> MKITNKSVDKQHIEKLDELRKNVSCTVIGFAEQTAELQQEISELFIAEFGVNGPIDMNSLSKLARITSYYASSEYFQGLAKYQRTACKMFITWQTLRKEAMECRSKDREIFASIPAKLCFFYFYNGELCRAVVCLLDYIDLSDDTLAKEAALRWLMFLGETELIEKKLKTWKMDKSSKDMFSATEFAMNYLKKSEYRVEMLEKLMKLRDKVKSDPTRSFSRYELASYVSWLCSTLSNVPVGSALRECEFPDRVSHIQEAALKSDSLVRNRIPGLASSQFDNSVNASIWPFLDGHQEDSNYYVHIGSTIAWHFEMRRECALVNVTTAQTRDSMSAMILNLRVALKSASFFRVLQTTNTLAYYSSIIEEAGSEK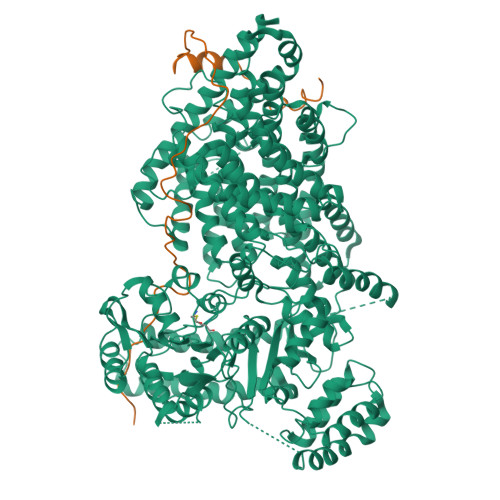NAKLMRVSCVNLLSSNPIIVRCSTPKETGATSRAHTPMAGSSVSEKQNTMRPDLADLLGDLELLDEQSFHPITRSCVCNVCTIYPLHSSFAAEYMMSYAIHSDFSQLSIKHFNDEFARIRERGMSSQVLMHRDSSVRPRPNIIQNEIFGMCVIRWLTKKLDSKESADEDTMEIFNNALKIVRYLQQRTTDMILAVTQLGRQLEFPMECNYSWMRPTIRKPRVKATIDCAVDILRAVSPFGRRPKVEKLEKNLQPFDKERFEKVRLAMRNEMNHYGHILYREWRCRLFAYVGRTSRDPWEAAYAWAESTQIGARNAVQSRLEKCKRGLVTMSGHDRFKTCVQSMPDEMTLVQIAMADDKTIYLVKLHADRDPIIMPLAHYSQAVELMDKFTFLLDEDEMIAKYPGDITPEEFWKRRKIVDGRMMTFVDEVQKHFLGVAASLLMPSGQLGPKAAELAIKIHKLSKGGLLLGEAKEMVYQSKLMDAKSWEALILRFCEMRTTDEKFKSFLPLMHRNSVEVMNQDDSIVTEKKYTYLVICPHLSQFCWERLPIFDEYPYVGRQVSIHSTFSQLEAMKSQEKQIPLQIDVQNAYYILDPDNNLGETQKRMVEYINKFNWEGTVGSAPKSNEISAALSQRDAFFFIGHGSGSSVMPRSVLKQSTCNAISLLMGCGSVRTIPQALGFDGKTAILDYAMAKCPLIVGCLWTVTDGEIDRFLIRMIDDCFEDSKSLTGIDKLRQLSEAMHEARSKARLKYLTGAAVVMYGLPVVAKQTTPFVEKDQRNLPQTPKTSARTSMRMETVPKTPKQEFVTSKSVPMTPIFSNNENKSPSRARMPSRVLKTPRQVKTFQEEDDEAPKRSTTRQLKPLVAPPIPATPTTRTTRSSARTPSRSRNL;> MEDLNFEERGSTQIPASLQQHFSAKLGRQNELEKTPSRGGLGLVVNSSKTPGGKSLQSLASACKVPPSTKKNTIPIAFECYEDETDDQIADVATIKKTEKHPCSPIDTANRCETFDSLAADIEDDMLNLEDQDVVLSEDRPYGDVIDPAESEAEALAELGVEEWDSYPPIDPASRIGDDFNYVLRTEDFAEEGDVKLEETRHRTVIADIDEVKMSKAERNELFSMLADDLDSYDLLAEEANLPL> KRAETLVFSTHAVISMRDGKLCLMFRVGDLRNSHIVEASIRAKLIKSKQTSEGEFIPLNQTDINVGYYTGDDRLFLVSPLIISH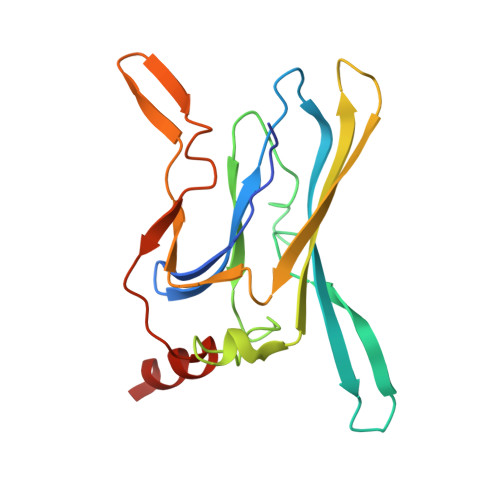EINQQSPFWEISKAQLPKEELEIVVILEGMVEATGMTCQARSSYITSEILWGYRFTPVLTLEDGFYEVDYNSFHETYETSTPSLSAKELAELANRAEL> GSHMASGAPPSVDLTSIQWRMPEWVQSMGGLRTENVLEYFSQSPFYSHKSNNEMLKMQSQFNALDLGDLNSQLKRLTGIQFVIIHERPPFLWVIQKQNRLNENEVKPLTVYFVCNENIYMAPNAYTLLATRMLNATYCFQKALTKIEKFPQYNPQEGYTYPKLSNDNLEVDHSNTNEPADENK;> MEDISTEKTVESLEAIRHRIAQIVQSLTHFLAILHQSESLSPWPTIHKNFNILLSQIHSLSNNLAAHSHTLQTTSIYPSLEFPVKEQEPLLTTLLRTKALPEVEEWEANTLQEYEASISSQPKKKEANDAYQKDQLWDQARIIFMEERENYSWFDFVTRRQESEGEFVSQRQLEIDRATEEQNANQMLTDILSFMKSGKR;> MTNSDDDLFSEKSTSSDTQQVQNILELEAKIPDILSSAGKCIEAIQLNNSLEDFRKYSKEFLETVEFISTGLRRQALELEKAEVPVVSLQPKKRYASTPLSNLIFDQSSKLM;> GNVLEFATLDSKRNVNDTEVESMDSQAYKKELIEQIMIAQTECSLALDMTSLLLSKFKENSIETISPFLKSTVPPSSLQFSRSQPPESKESDATLAKCWKEKSLTSSCKFLFEAKERLTSVVETEHEYYTELVKVKEASWPLFNSQGSNHLSVQYSCLGGISLGLGLIRMKPESKSFEVQSSLLYSQAALKISILNKDRDEIGSSTWSWPSQNCNSVLLKDIYKLQEILFEMDIWNSLLQEAQSCGNQGVNFTGDEILVPISDDHVVRITLETSSKNTESGFTEDKKSNEDTSTNFVTIKQEKELLKCLCDTLNAIAHILFLKHCRKSDRRSQQPELYMAIDANAPLILRPLIFYYNLNQESLEFQRWLKQRDISFKFMPNYPWEKAKDFLELENSLSINRLSISWRIMVSNFEPAIFIQHTPTLHGTDKSVWRCKDQYSSNQFSSLKNVCQYIEHHINSLSRRSKKTE;> ASMQELYLLGVVPSRRFEAVVNSLSKTLDGPKTILEFWVVYRPKDVPPNLPRQPDSWLRLCSNIESHDETDTEWSKNTQWSMYLEGNSEPK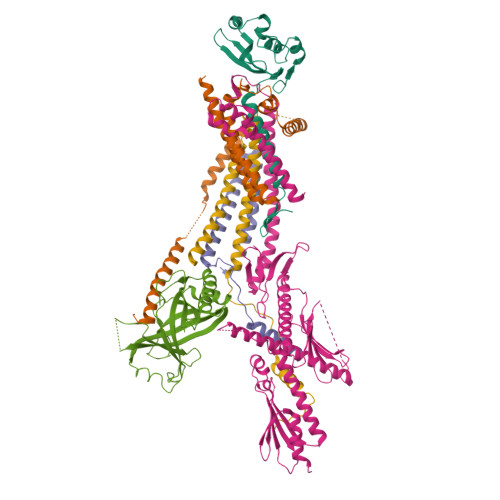REDKCGIRPVNRAKLTNGSVTEFVEKMGYEFSHEYIIQGLEYFFFDTTVRIYQTLIPSQQRSIKPPFHPMNEEQPWILHVYTHVADASNQVAMAKAEANLTKVKTLLSAFCDLKNVRL;> SSDSFQRQLVQRTNTLNSSIDNATLTILSRFQDILDIAINEGKDKYTVAPEVYQIECHTVSMVRAVEQLLDVSRQIKSYWLTNSLSTSFPTVDYSEPDLEKVKRTLTKLQNHLLEVSLIEPEASETTEAPTVSDT> MPQSKSRKIAILGYRSV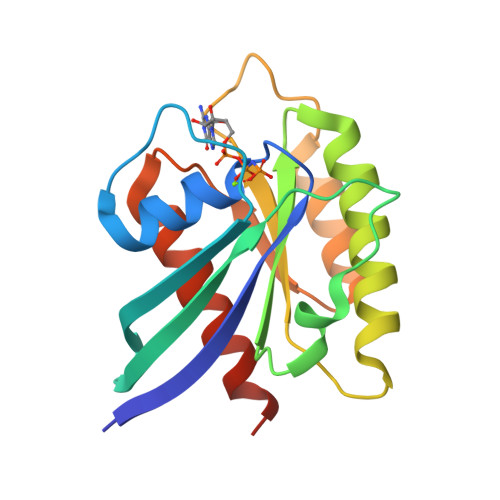GKSSLTIQFVEGQFVDSNDPTIENTFTKLITVNGQEYHLQLVDTAGQDEYSIFPQTYSIDINGYILVYSVTSIKSFEVIKVIHGKLLDMVGKVQIPIMLVGNKKDLHMERVISYEEGKALAESWNAAFLESSAKENQTAVDVFRRIILEAEKLEHHHHHH>GSHMEQLKHCNGILKELLSKKHAAYAWPFYKPVDASALGLHDYHDIIKHPMDLSTVKRKM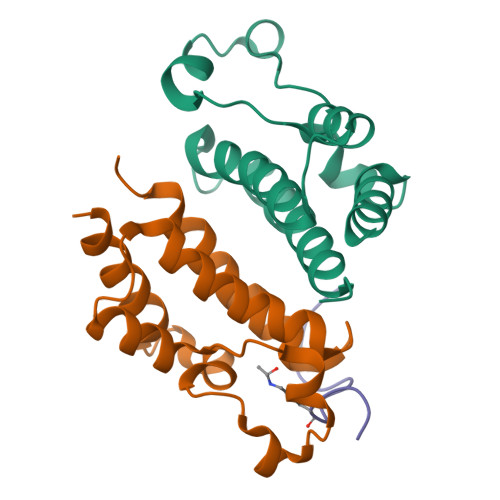ENRDYRDAQEFAADVRLMFSNCYKYNPPDHDVVAMARKLQDVFEFRYAKMPD[4x];>[2x]SGRGKGGKGLGKGGA> SNAEATLGSGNLRQAVMLPEGEDLNEWIAVNTVDFFNQINMLYGTITEFCTEASCPVMSAGPRYEYHWADGTNIKKPIKCSAPKYIDYLMTWVQDQLD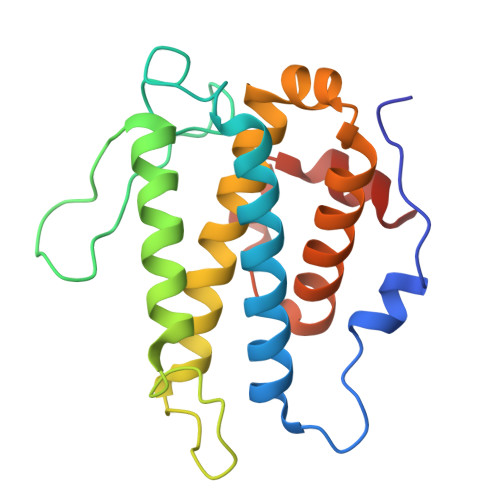DETLFPSKIGVPFPKNFMSVAKTILKRLFRVYAHIYHQHFDSVMQLQEEAHLNTSFKHFIFFVQEFNLIDRRELAPLQELIEKLGSKDR> ASVDFKTYVDQACRAAEEFVNVYYTTMDKRRRLLSRLYMGTATLVWNGNAVSGQESLSEFFEMLPSSEFQISVVDCQPV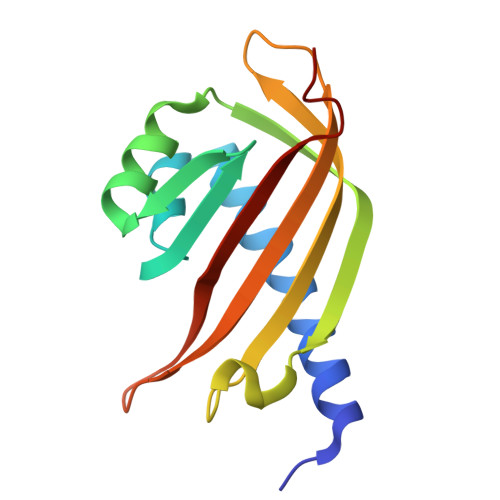HDEATPSQTTVLVVICGSVKFEGNKQRDFNQNFILTAQASPSNTVWKIASDCFRFQDWAS> GGUCGGGUAGUGAGGGCCUUGGUCAGACGCAGCGGGCGUGCUUGUGGACUGCUUGGUGGGGCUUGCUCUGCUAGGCGGACUACUUGCGUGCCUUGUUGUAGACGGCCUUGG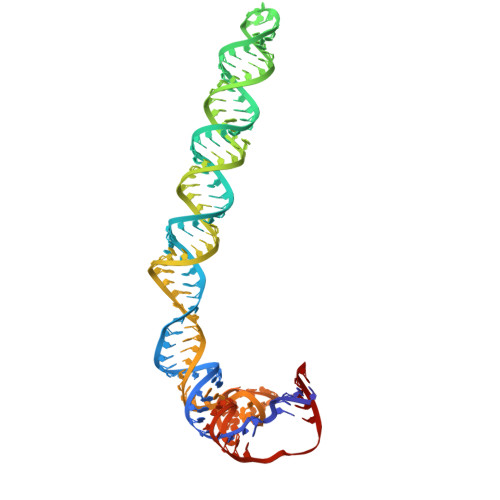UAGGUCUCUUGUAGACCGUCGCUUGCUACAAUUAACGAUC>MAHAGRTGYDNREIVMKYIHYKLSQRGYEWDAGDVGAAPPGAAPAPGIFSSQPGHTPHPAASRDPVARTSPLQTPAAPGAAAGPALSPVPPVVHLTLRQAGDDFSRRYRRDFAEMSSQLHLTPFTARGRFATVVEELFRDGVNWGRIVAFFEFGGVMCVESVNREMSPLVDNIALWMTEYLNRHLHTWIQDNGGWDAFVELYGPSMRLEHHHHHH[2x];>MADPKKVLDKAKDEAENRVRELKQRLEELYKEARKLDLTQEMRQELVDKARAASLQANGDIFYAILRALAEAEKL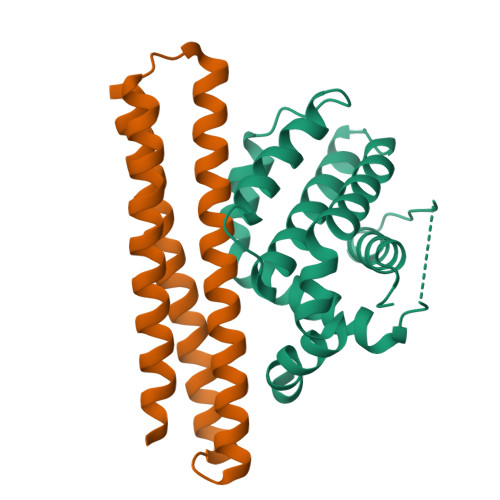KKAGLVNSQQLDELKRRLEELAEEARRKAEKLRDEFRLKLEYG[2x]>[4x]GPMVSEQSEIVTSKYQKIAVAVAQRIANGDYEVGEKLKSRTTIASTFNVSPETARKGLNILADLQILTLKHGSGAIILSKEKAIEFLNQYETS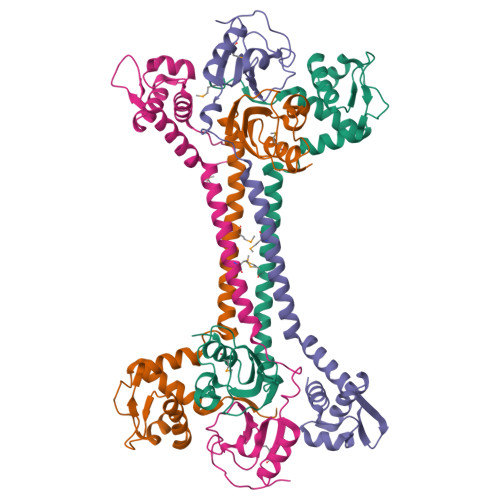HSVAILKGKIRDNIKAQQQEMEELATLVDDFLLQTRAVSKQYPLAPYEIIVSEDSEHLGKSIGELNVWHQTGATIVAIEHEGKFIVSPGPFSVIEQGDHIFFVGDEDVYARMKTYFNLRMGL>MSCYIYWDKIKRIASRLEGMNYHFDEMDTSGVMPLLDEIEEIAHDSTIDFESAKHILDDAEMNHALSLIRKFYVNLGMKLQMEKAQEVIESDSPWETLRSFYFYPRYLELLKNEAALGRFRRGERAVFIGGGPLPLTGILLSHVYGMRVNVVEIEPDIAELSRKVIEGLGVDGVNVITGDETVIDGLEFDVLMVAALAEPKRRVFRNIHRYVDTETRIIYRTYTGMRAILYAPVSDDDITGFRRAGVVLPSGKVNNTSVLV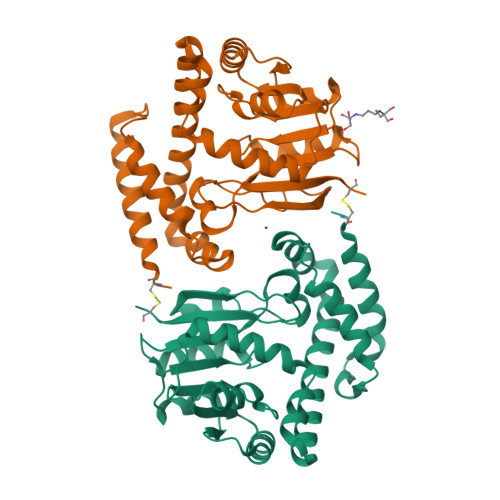FKCPDKGELNSKLEGKPIPNPLLGLDSTRTGHHHHHH[2x]>MASKKVCIVGSGNWGSAIAKIVGGNAAQLAQFDPRVTMWVFEEDIGGKKLTEIINTQHENVKYLPGHKLPPNVVAVPDVVQAAEDADILIFVVPHQFIGKICDQLKGHLKANATGISLIKGVDEGPNGLKLISEVIGERLGIPMSVLMGANIASEVADEKFCETTIGCKDPAQGQLLKELMQTPNFRITVVQEVDTVEICGALKNVVAVGAGFCDGLGFGDNTKAAVIRLGLMEMIAFAKLFCSGPVSSATFLESCGVADLITTCYGGRNRKVAEAF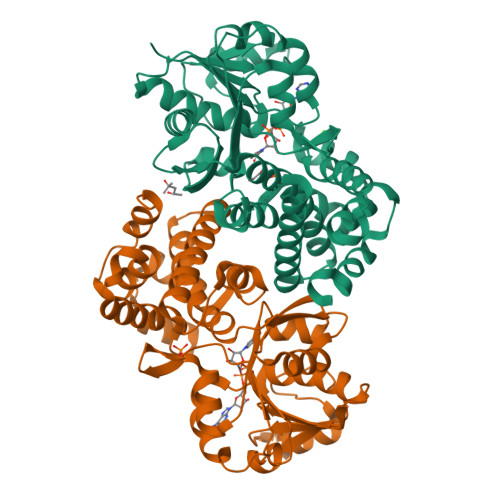ARTGKSIEQLEKELLNGQKLQGPETARELYSILQHKGLVDKFPLFMAVYKVCYEGQPVGEFIHCLQNHPEHM[4x]> MGHHHHHHENLYFQMNTPTDLKVTKRDGRLEAIDLDKIHRVVTWAAEGLENVSVSQVELKSHIQFYNGIRTDDIHETIIKAAADLISEDTPDYQYLAARLAIFHLRKIAYGEYEPPHLYNHVKKLTDAGKYDRHILEDYSREEFDELNAYIDHERDMSFSYAAVKQLEGKYLVQNRVTRQIYETPQFLYVLVAMCLFSKYPKEARLDYVKRFYDAVSTFKVSLPTPIMSGVRTPTRQFSSCVLIECDDSLDSINATTSAIVKYVSQRAGIGINAGRIRGLDSEIRGGEARHTGCIPFFKMFQAAVKSCSQGGVRGGAATLFYPLWHIEAESLLVLKNNRGVEDNRIRQLDYGVQINRLLYTRLIKGGNITLFSPNEVSGLYEAFFADQDEFERLYTKYEQDPNIRKRIIPAADLFSTLMQERAGTGRIYIQNVDHCNTHSPFDPRVAPVHQSNLCMEIALPTKPLDNINDPDGEIALCTLSAFNLGALNSLD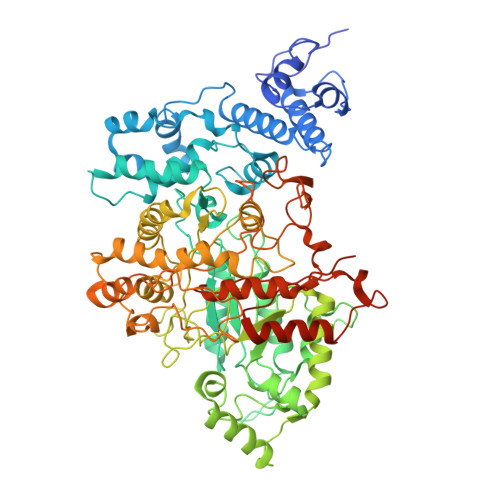ELEGLADLTVRALDALLDYQGYPVEAARTSTMDRRSLGIGVINYAYYLAKNGVRYSDGSALGLTHRTFEAIQYYLLKASANLAKEYGACTLFNQTVYSQGKLPIDTYKKDLDAVCGEPLHYDWESLRADIVKYGLRNSTLTALMPSETSSQIANATNGIEPPRGLVTVKASKDGILKQVVPEFETLKNAYETLWQLPGNEGYLKLVGVMQKFVDQAISANTAYDPGKFEGNKVSMKQMLKDLLTAYKYGVKTLYYHNTRDGADDTQTDIQDDGCAGGACKI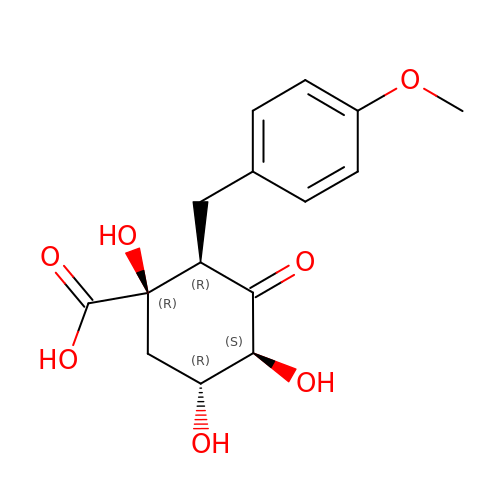(1R,2R,4S,5R)-1,4,5-TRIHYDROXY-2-(4-METHOXYBENZYL)-3-OXOCYCLOHEXANECARBOXYLIC ACID | C15 H18 O7 | KDOXKRDIRCHNDT-YODMDTAWSA-N4-amino-8-methylpteridine-2,7(1H,8H)-dione | C7 H7 N5 O2 | 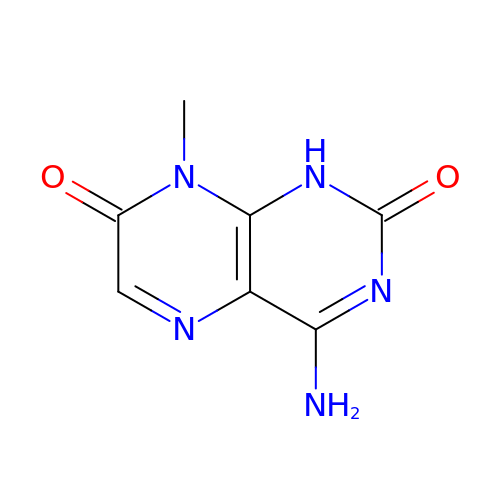IIYMXMJOUCDTSZ-UHFFFAOYSA-N>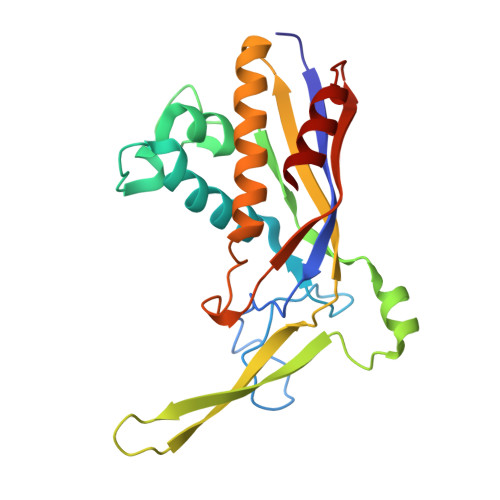 MTFAKIKFSAQIRLETGLHIGGSDAFAAIGAIDSPVIKDPITNLPIIPGSSLKGKMRTLLAKVYNEKVAEKPSDDSDILSRLFGNSKDKRFKMGRLIFRDAFLSNADELDSLGVRSYTEVKFENTIDRITAEANPRQIERAIRNSTFDFELIYEITDENENQVEEDFKVIRDGLKLLELDYLGGSGSRGYGKVAFENLKATTVFGNYDVKTLNELLTAEV Sclerotium rolfsii lectin (SRL) is a cell wall-associated developmental–stage specific lectin secreted from the soil–born pathogenic fungus. SRL displays a clear specificity for TF and its substituted glycan structures. In the current study we report two recombinant variants SSR1 and SSR2, generated by the deliberate changes of the amino acids incorporated at particular sites of SRL by the synthetic gene construct method based on the complete amino acid sequence of SRL. Interestingly, SSR1 and SSR2 the two different variants of SRL, differ in their glycan specificity.

In both the SSR1-GlcNAc and the SSR2-GlcNAc complexes, determined at 1.9 Å and 1.7 Å respectively, GlcNAc was found bound only in the secondary carbohydrate binding site of SRL in agreement with the complex of GlcNAc with SRL. In the SSR1-GlcNAc structure an MPD molecule was found bound in the primary carbohydrate binding site similarly to the SRL-GlcNAc complex structure. All atoms of the ligand are well defined in both variant complexes, within the electron density map which has shown that GlcNAc binds to this site with two alternative conformations with respect to the hydroxyl group O1, α and β that have equal occupancies. The rms displacement values for all atoms upon superposition of the SSR1-GlcNAc and the SSR2-GlcNAc structures onto the SRL-GlcNAc structure are 0.5 Å and 0.4 Å, respectively. The structural mode of binding of GlcNAc does not differ significantly in the variants and the SRL structure. Briefly, GlcNAc is involved in hydrogen bond interactions with residues Asp77, Ile78, Thr80, Arg101, and Tyr112. All hydroxyl groups of GlcNAc except hydroxyl group O1, are involved in hydrogen bond interactions with protein residues, a fact that offers an explanation for the alternative conformations of this group. In both alternative conformations, the hydroxyl group O1, in the ligand complexes, is involved in hydrogen bond interactions only with water molecules. The glycan array analysis of the variants demonstrated that SSR1 recognizes TF antigen and its derivatives with high affinity like SRL but showed the highest affinity towards the sialylated Tn antigen, unlike SRL.

>TYKITVRVYQTNPDAFFHPVEKTVWKYANGGTWTITDDQHVLTMGGSGTSGTLRFHADNGESFTATFGVHNYKRWCDIVTNLAADETGMVINQQYYSQKNREEARERQLSNYQVKNAKGRNFQIVYTEAEGNDLHANLIIG[2x]>MGSSGKLADCTAQDLNRTELFLVEGDSAGGSAKQARDREYQAIMPLKGKILNTWEVSSDEVLASQEVHDISVAIGIDPDSDDLSQLRYGKICILADADSDGLHIATLLCALFVRHFRTLVKEGHVYVALPPLYRIDLGKEVYYALTEEEKTGVLEQLKRKKGKPNVQRFKGLGEMNPMQLRETTLDPNTRRLVQLVISDEDEQQTTAIMDMLLAKKRSEDRRNWLQEKGDMADLEVESMSDMAERLALHEFTENAYLNYSMYVIMDRALPFIGDGLKPVQRRIVYAMSELGLNASAKFKKSARTVGDVLGKYHPHGDSACYEAMVLMAQPFSYRYPLVDGQGNWGAPDDPKSFAAMRYTESRLSKYAELLLSELGQGTVDWVPNFDGTLQEPKMLPARLPNILLNGTTGIAVGMATDIPPHNLREVAKAAITLIEQPKTTLDELLDIVQGPDFPTEAEIITSRAEIRKIYQNGRGSVRMRAVWSKEDGAVVISALPHQVSGAKVLEQIAAQMRNKKLPMVDDLRDESDHENPTRLVIVPRSNRVDMEQVMNHLFATTDLEKSYRINLNMIGLDGRPAVKNLLEILSEWLVFRRDTVRRRLNHRLEKVLKRLHILEGLLVAFLNIDEVIEIIRTEDEPKPALMSRFGISETQAEAILELKLRHLAKLEEMKIRGEQSELEKERDQLQAILASERKMNNLLKKELQADADAFGDDRRSPLHEREEAKALEHHHHHH[4x]

DNA gyrase and topoisomerase IV are essential, homologous, highly conserved bacterial type II topoisomerases and are established targets of many successful antibiotics. These enzymes resolve topological challenges during DNA replication and transcription. BWC0977 is a pyrazino-oxazinone based novel bacterial topoisomerase inhibitor (NBTI) currently in Phase 1 clinical trials and demonstrates potent activity against multidrug-resistant Gram-negative and Gram-positive bacteria. It targets both DNA gyrase and topoisomerase IV with balanced low-nanomolar potencies, showing remarkable superiority over ciprofloxacin and gepotidacin.

While structural analyses confirm NBTI interactions with DNA gyrases, the interactions with topoisomerase IV remain speculative. This study reports the first structural analysis of K. pneumoniae topoisomerase IV complexed with BWC0977 at 3.05 Å resolution, alongside biochemical characterization revealing its potent and balanced dual-targeting mechanism. The asymmetric unit contains two copies of the ParEC-core dimer, each bound to double-stranded DNA and BWC0977. Unbiased electron density maps identified a single BWC0977 molecule intercalated between DNA bases at positions +2 and +3 (between A and T base pairs), forming a stable topoisomerase IV–DNA–BWC0977 ternary complex. The 7-Fluoro-1-methylquinolin-2(1H)-one ring (LHS) of BWC0977 intercalates between DNA bases, engaging in π–electron interactions. The right-hand side (RHS) of BWC0977 consists of pyrazino-oxazinone and oxazolidinone moieties, which interact with key residues D79, M118, and R119 of ParC. The -NH group of the pyrazino-oxazinone moiety forms a hydrogen bond with the ParC D79 from one subunit, while the oxazolidinone nitrogen interacts with the catalytically important R119 and while maintaining a weak interaction with the D79 from the second ParC subunit. These interactions stabilize the closed DNA gate conformation, effectively inhibiting the topoisomerase IV activity. Further stabilization arises from π–sulfur interactions between M118 and the pyrazino-oxazinone moiety. Structural comparisons between BWC0977 and gepotidacin reveal that the oxazolidinone ring of BWC0977 forms two to three additional hydrogen bonds with the R119 side chain guanidino group as well as the main chain NH.> MEQQPLTLTAATTRAQELRKQLNQYSHEYYVKDQPSVEDYVYDRLYKELVDIETEFPDLITPDSPTQRVGGKVLSGFEKAPHDIPMYSLNDGFSKEDIFAFDERVRKAIGKPVAYCCELKIDGLAISLRYENGVFVRGATRGDGTVGENITENLRTV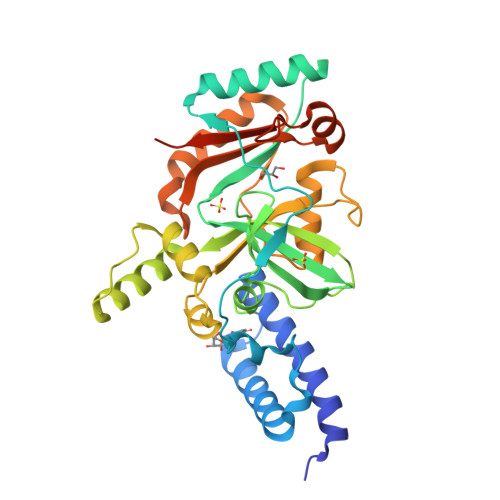RSVPMRLTEPISVEVRGECYMPKQSFVALNEEREENGQDIFANPRNAAAGSLRQLDTKIVAKRNLNTFLYTVADFGPMKAKTQFEALEELSAIGFRTNPERQLCQSIDEVWAYIEEYHEKRSTLPYEIDGIVIKVNEFALQDELGFTVKAPRWAIAYKFPPEEAETVVZHHHHHH> ACTKNAIAQTGFNKDKYFNGDVWY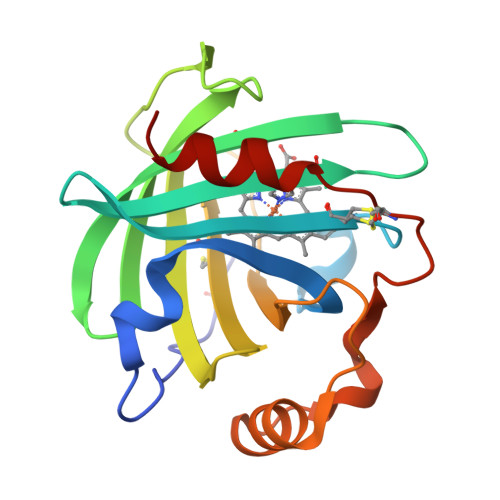VTDYLDLEPDDVPKRYCAALAAGTASGKLKEALYHYDPKTQDTFYDVSELQVESLGKYTANFKKVDKNGNVKVAVTAGNYYTFTVMYADDSSALIHTCLHKGNKDLGDVYAVLNRNKDAAAGDKVKSAVSAATLEFSKFISTKENNCAYDNDSLKSLLTK>[2x]MDAEYDLKFGMNAGTSSNEYKAAEMFAKEVKEKSNGKIEISLYPSSQLGDDRAMLKQLKDGALDFTFAESARFQLFYPEAAVFALPYVITNYEVAQ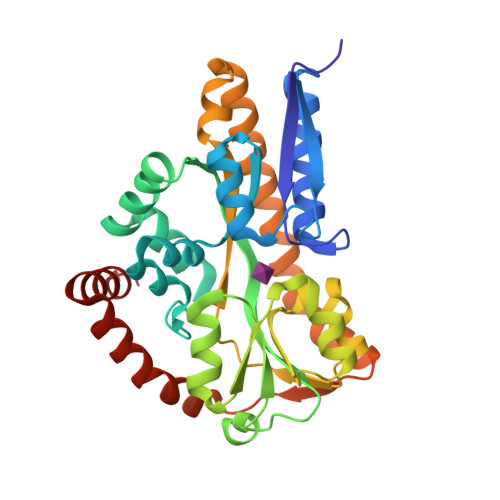KALHDTAFGKDLIQKMNKELGLTLLSQAYNGTRQTTSNRAINGIADMKGLKLRVPNAATNLAYAKYVGASPTPMAFSEVYLALQTNSVDGQENPLATVQAQKFYEVQKYLAITNHILNDQLYLVSSETFADLPEDLQKVVKKAAQKAAEYHTKLFVDGEKELVTFFEKQGVTVTHPDLTPFKDAMKPYYAEFVKQTGAKGEEVLKQIQAINK> GPGSGFGTSPLTPSARISALNIVGDLLRKVGALESKLAAC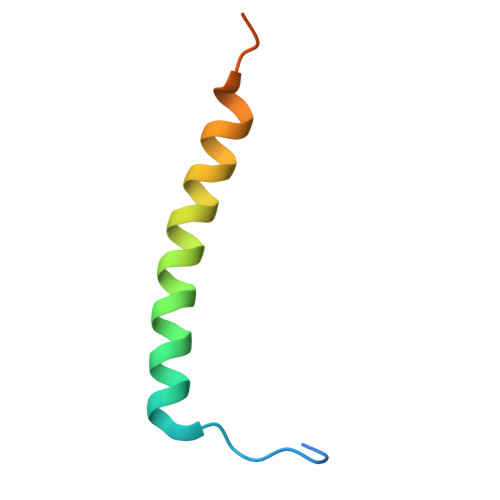RNFAKDQASRK> GSGPEEEFGMSLIKHNSCVITTENGKFTGLGVYDRFVVVPTHADPGKEIQVDG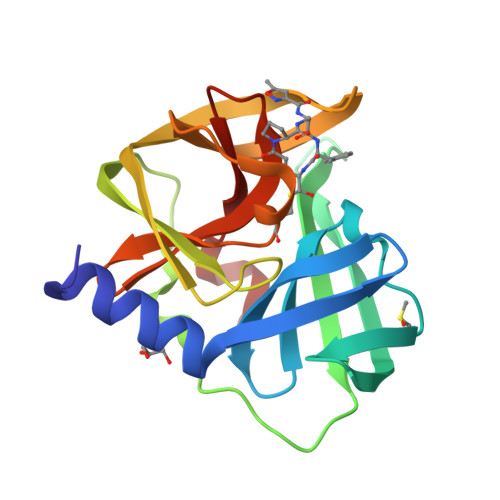ITTKVIDSYDLYNKNGIKLEITVLKLDRNEKFRDIRRYIPNNEDDYPNCNLALLANQPEPTIINVGDVVSYGNILLSGNQTARMLKYSYPTKSGYCGGVLYKIGQVLGIHVGGNGRDGFSAMLLRSYFT[(2~{R},3~{S},4~{R},5~{R})-5-(2-azanyl-6-oxidanylidene-3~{H}-purin-9-yl)-3,4-bis(oxidanyl)oxolan-2-yl]methoxy-~{N}-ethyl-phosphonamidic 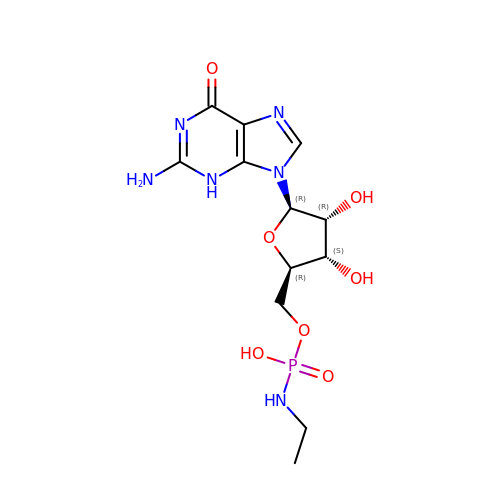acid | C12 H19 N6 O7 P | BTIPXEHUJHIGFX-IOSLPCCCSA-N> MQRKAKLQEFKRAQKAENLLKLAAEKLGKDFETAWREVWVPLEEEWGEVYAAFEDAAKDGIDVLKGHVPDEWLPVLKEIIDNYVEVPTVTIDAEFEITVPKPNGVEIIKEALIRARDRANKEKDVEVKFTYLGAPRYRIDITAPDY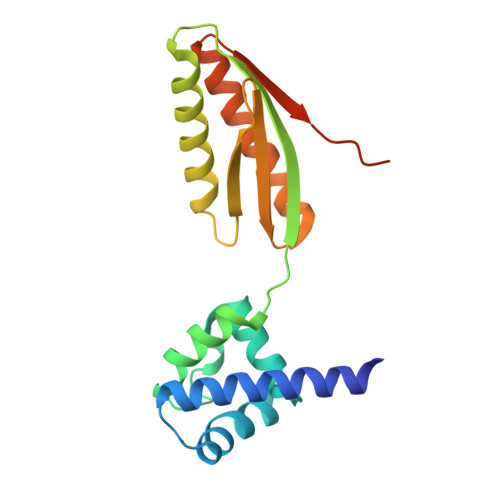YKAEEVLESIAEEILRVIKEAGGEATLLRKEKRIKKVKKRKK>[2x]ARLGARPCGLRELEVRVSELGLGYASDETVLFRYCAGACEAAARVYDLGLRRLRQRRRLRRERVRAQPCCRPTAYEDEVSFLDAHSRYHTVHELSARECACV;>SSLQGPELHGWRPPVDCVRANELCAAESNCSSRYRTLRQCLAGRDRNTMLANKECQAALEVLQESPLYDCRCKRGMKKELQCLQIYWSIHLGLTEGEEFYEASPYEPVTSRLSDIFRLASIFSGTGADPVVSAKSNHCLDAAKACNLNDNCKKLR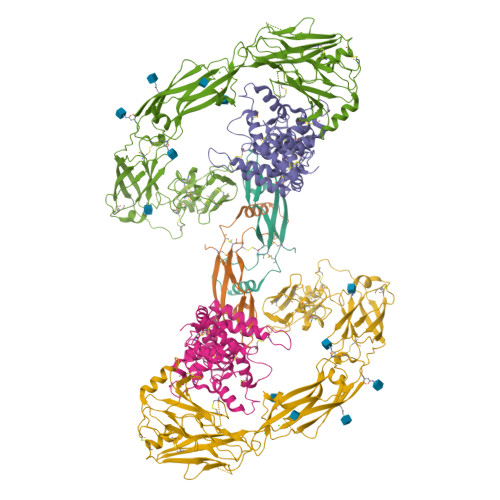SSYISICNREISPTERCNRRKCHKALRQFFDRVPSEYTYRMLFCSCQDQACAERRRQTILPSCSYEDKEKPNCLDLRGVCRTDHLCRSRLADFHANCRASYQTVTSCPADNYQACLGSYAGMIGFDMTPNYVDSSPTGIVVSPWCSCRGSGNMEEECEKFLRDFTENPCLRNAIQAFGNGTDVNGTHHHHHHHH[2x];>[2x]LYFSRDAYWEKLYVDQAAGTPLLYVHALRDAPEEVPSFRLGQHLYGTYRTRLHENNWICIQEDTGLLYLNRSLDHSSWEKLSVRNHGFPLLTVYLKVFLSPTSLREGECQWPGCARVYFSFFNTSFPACSSLKPRELCFPETRPSFRIRENRPPGTFHQFRLLPVQFLCPNISVAYRLLEGEGLPFRCAPDSLEVSTRWALDREQREKYELVAVCTVHAGAREEVVMVPFPVTVYDEDDSAPTFPAGVDTASAVVEFKRKEDTVVATLRVFDADVVPASGELVRRYTSTLLPGDTWAQQTFRVEHWPNETSVQANGSFVRATVHDYRLVLNRNLSISENRTMQLAVLVNDSDFQGPGAGVLLLHFNVSVLPVSLHLPSTYSLSVSRRARRFAQIGKVCVENCQAFSGINVQYKLHSSGANCSTLGVVTSAEDTSGILFVNDTKALRRPKCAELHYMVVATDQQTSRQAQAQLLVTVEGSYVAEEAGCPLSCAVSKRRLECEECGGLGSPTGRCEWRQGDGKGITRNFSTCSPSTKTCPDGHCDVVETQDINICPQDCLRGSIVGGHEPGEPRGIKAGYGTCNCFPEEEKCFCEPEDIQDPLCDELCRGTHHHHHHHH>MSGGDGRGHNTGAHSTSGNINGGPTGLGVGGGASDGSGWSSENNPWGGGSGSGIHWGGGSGHGNGGGNGNSGGGSGTGGNLSAVAAPVAFGFPALSTPGAGGLAVSISAGALSAAIADIMAALKGPFKFGLWGVALYGVLPSQIAKDDPNMMSKIVTSLPADDITESPVSSLPLDKATVNVNVRVVDDVKDERQNISVVSGVPMSCPVVDAKPTERPGVFTASIPGAPVLNISVNNSTPAVQTLSPGVTNNTDKDVRPAGFTQGGNTRDAVIRFPKDSGHNAVYVSVSDVLSPDQVKQRQDEENRRQQEWDATHPVEAAERNYERARAELNQANEDVARNQERQAKAVQVYNSRKSELDAANKTLADAIAEIKQFNRFAHDPMAGGHRMWQMAGLKAQRAQTDVNNKQAAFDAAAKEKSDADAALSSAMESRKKKEDKKRSAENNLNDEKNKPRKGFKDYGHDYHPAPKTENIKGLGDLKPGIPKTPKQNGGGKRKRWTGDKGRKIYEWDSQHGELEGYRASDGQHLGSFDPKTGNQLKGPDPKRNIKKYL[2x];>[2x]GLKLDLTWFDKSTEDF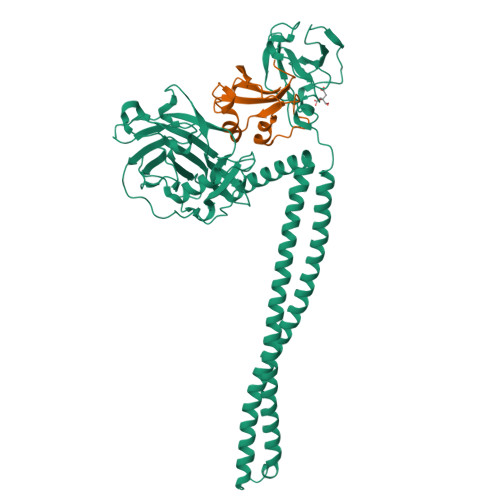KGEEYSKDFGDDGSVMESLGVPFKDNVNNGCFDVIAEWVPLLQPYFNHQIDISDNEYFVSFDYRDGDW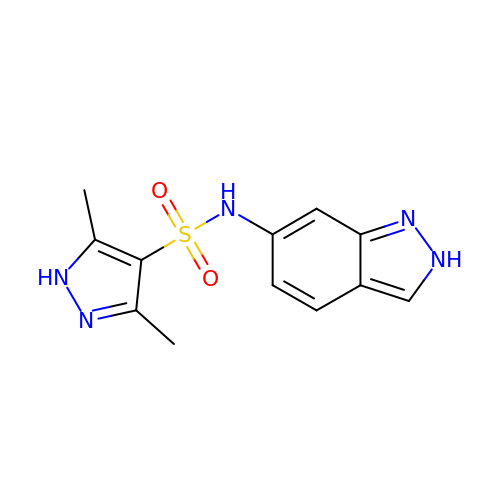~{N}-(2~{H}-indazol-6-yl)-3,5-dimethyl-1~{H}-pyrazole-4-sulfonamide | C12 H13 N5 O2 S | ZPEANOFCXGJMGS-UHFFFAOYSA-N>PISPIETVPVKLKPGMDGPKVKQWPLTEEKIKALVEICTEMEKEGKISKIGPENPYNTPVFAIKKKDSTKWRKLVDFRELNKRTQDFWEVQLGIPHPAGLKKKKSVTVLDVGDAYFSVPLDEDFRKYTAFTIPSINNETPGIRYQYNVLPQGWKGSPAIFQSSMTKILEPFKKQNPDIVIYQYMDDLYVGSDLEIGQHRTKIEELRQHLLRWGLTTPDKKHQKEPPFLWMGYELHPDKWTVQPIVLPEKDSWTVNDIQKLVGKLNWASQIYPGIKVRQLSKLLRGTKALTEVIPLTEEAELELAENREILKEPVHGVYYDPSKDLIAEIQKQGQGQWTYQIYQEPFKNLKTGKYARMRGAHTNDVKQLTEAVQKITTESIVIWGKTPKFKLPIQKETWETWWTEYWQATWIPEWEFVNTPPLVKLWYQLEKEPIVGAETFYVDGAANRETKLGKAGYVTNKGRQKVVPLTNTTNQKTELQAIYLALQDSGLEVNIVTNSQYALGIIQAQPDKSESELVNQIIEQLIKKEKVYLAWVPAHKGIGGNEQVDKLVSAG[2x];>[2x]GPISPIETVPVKLKPGMDGPKVKQWPLTEEKIKALVEICTEMEKEGKISKIGPENPYNTPVFAIKKKDSTKWRKLVDFRELNKRTQDFWEVQLGIPHPAGLKKKKSVTVLDVGDAYFSVPLDEDFRKYTAFTIPSINNETPGIRYQYNVLPQGWKGSPAIFQSSMTKILEPFKKQNPDIVIYQYMDDLYVGSDLEIGQHRTKIEELRQHLLRWGLTTPDKKHQKEPPFLWMGYELHPDKWTVQPIVLPEKDSWTVNDIQKLVGKLNWASQIYPGIKVRQLSKLLRGTKALTEVIPLTEEAELELAENREILKEPVHGVYYDPSKDLIAEIQKQGQGQWTYQIYQEPFKNLKTGKY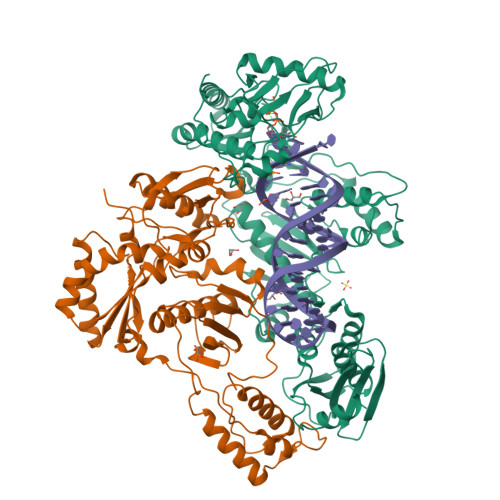ARMRGAHTNDVKQLTEAVQKITTESIVIWGKTPKFKLPIQKETWETWWTEYWQATWIPEWEFVNTPPLVKLWYQ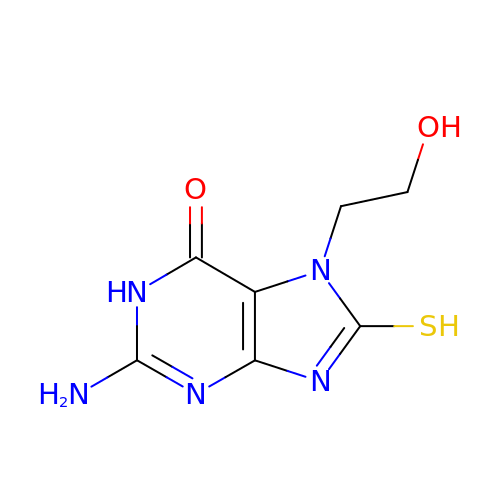7-(2-HYDROXYETHYL)-8-MERCAPTOGUANINE | C7 H9 N5 O2 S | OYFBJNRCXXDVIZ-UHFFFAOYSA-N>[2x]MEAAQAFENLANLEQEFGKAEIEILKKQNELFQPLFEQRRDILKTINNFWVVVLEAAGDEISQYITPEDSVLLEKLENIYVERFNEKEPRDVRISLTFQPNEYLQDDNLTL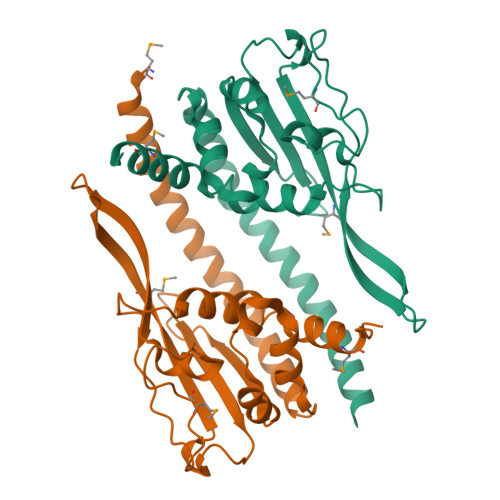VKEVRMKEEKAKDDEGLEKKITKYTSQPVDIHWKPGKSMFRKNKKLPPNFFDYFQWTGEEEDDDFDGATLTIFLAEDLFPNAVKYFTEAMTEEASDEDESVDLEEDEEEEDEEDEEGDEEKQEPPSKKSKKSNAAAENLYFQGLEDYKDDDDKHHHHHHHHHH> MAAQNEQRPERIKTTPYLEGDVLSSDSGPLLSVFALQEIMQKVRQVQADYMTATREVDFTVPDVQQILDDIKALAAEQVYKIVKVPSTSFRHIVTQSRDRVLRVDTYYEEMSQVGDVITEDEPEKFYSTIIKKVRFIRGKGSFILHDIPARDHRGMEVAEPEVLGVEFKNVLPVLTAEHRAMIQNALDGSIIENGNVATRDVDVFIGACSEPIYRIYNRLQGYIEAVQLQELRNSIGWLERLGQRKRITYSQEVLTDFRRQDMIWVLALQLPVNPQVVWDVPRSSIANLIMNIATCLPTGEYIAPNPRISSITLTQRITTTGPFAILTGSTPTAQQLNDVRKIYLALMFPGQIILDLKIDPGERMDPAVRMVAGVVGHLLFTA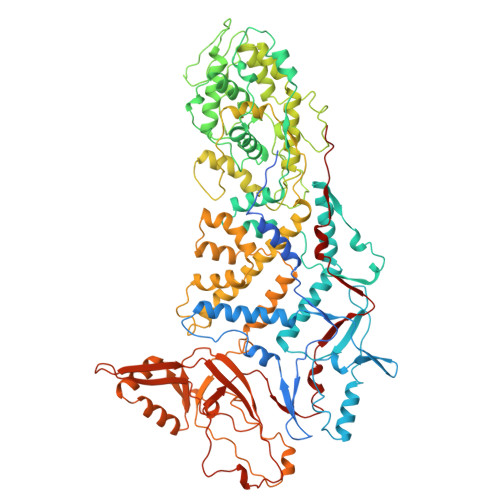GGRFTNLTQNMARQLDIALNDYLLYMYNTRVQVNYGPTGEPLDFQIGRNQYDCNVFRADFATGTGYNGWATIDVEYRDPAPYVHAQRYIRYCGIDSRELINPTTYGIGMTYHCYNEMLRMLVAAGKDSEAAYFRSMLPFHMVRFARINQIINEDLHSVFSLPDDMFNALLPDLIAGAHQNADPVVLDVSWISLWFAFNRSFEPTHRNEMLEIAPLIESVYASELSVMKVDMRHLSLMQRRFPDVLIQARPSHFWKAVLNDSPEAVKAVMNLSHSHNFINIRDMMRWVLLPSLQPSLKLVLEEEAWAAANDFEDLMLTDQVYMHRDMLPEPRLDDIERFRQEGFYYTNMLEAPPEIDRVVQYTYEIARLQANMGQFRAALRRIMDDDDWVRFGGVLRTVRVKFFDARPPDDILQGLPFSYDTNEKGGLSYATIKYATETTIFYLIYNVEFSNTPDSLVLINPTYTMTKVFINKRIVERVRVGQILAVLNRRFVAYKGKMRIMDITQSLKMGTKLAAPTV> MASLTVKAYLLGKEDAAREIRRFSFCCSPEPEAEAEAAAGPGPCERLLSRVAALFPALRPGGFQAHYRDEDGDLVAFSSDEELTMAMSYVK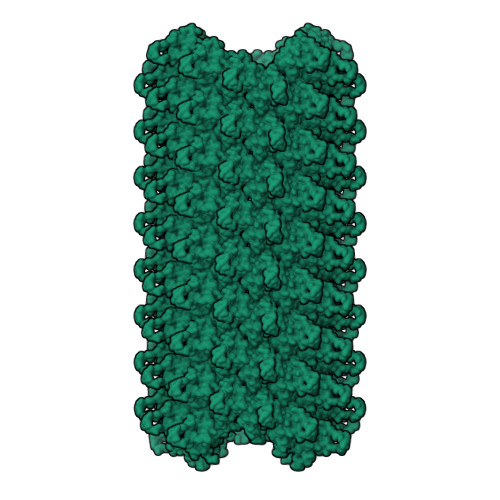DDIFRIYIKEKKECRRDHRPPCAQEAPRNMV N-{3-[(4-{[3-(TRIFLUOROMETHYL)PHENYL]AMINO}PYRIMIDIN-2-YL)AMINO]PHENYL}CYCLOPROPANECARBOXAMIDE | C21 H18 F3 N5 O | 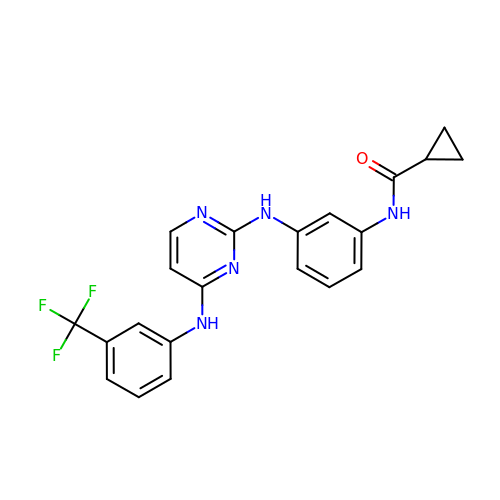RDTDWGQDFJPTPD-UHFFFAOYSA-N>[2x]MPKVKSGAIGRRRGRQEQRRELKSAGGLMFNTGIGQHILKNPLIINSIIDKAALRPTDVVLEVGPGTGNMTVKLLEKAKKVVACELDPRLVAELHKRVQGTPVASKLQVLVGDVLKTDLPFFDTCVANLPYQISSPFVFKL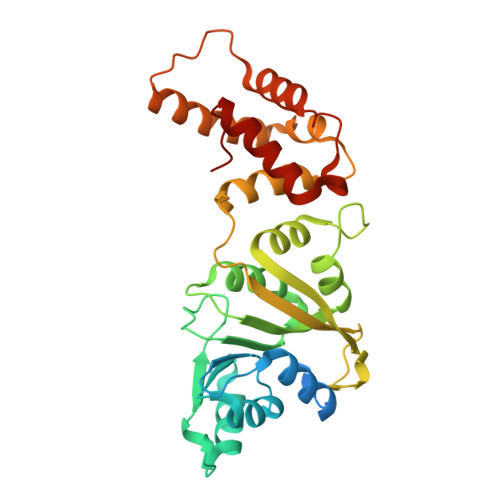LLHRPFFRCAILMFQREFALRLVAKPGDKLYCRLSINTQLLARVDHLMKVGKNNFRPPPKVESSVVRIEPKNPPPPINFQEWDGLVRITFVRKNKTLSAAFKSSAVQQLLEKNYRIHCSVHNIIIPEDFSIADKIQQILTSTGFSDKRARSMDIDDFIRLLHGFNAEGIHFS>[2x]SCSKCRKEMGQ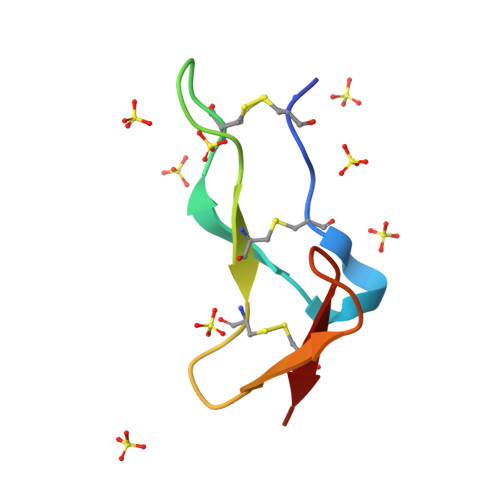VEISSCTVDRDTVCGCRKNQYRHYWSENLFQCFN>[2x]MANDSVSLTSNISNTSGVLLESQTKITDGALHFDGKKLNHNTFENPSKSQAYDYFFGRNISAHGDAVKPYKHFVFMTWYKGGKEERNVMLSRFNTKTGVVKTIQFPHRHTGFRGDPLVGESHNTIGLAVSPLNGTIHMVYDMHAYVDDDETGRFKGRFVDDFFRYSFSVAGAADVPDDEFTLEQFVKD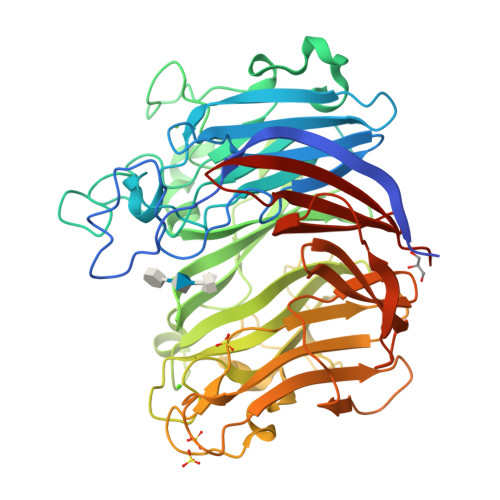TSELSQGADDYKHLTMTGNLQDKENFSALTYPKFYTSDDGELLHYMRWGGNNNGAYYFNKYDAKNQKWTRFTPFNHKDQKTHGNAYNWGLYGQMKYINGKLRVGFQQNSANNDDRFKYQNGVYYAYSDHPDGLGNWKNVDGEDMTWPLVNSDEIKIFEPGDYIDHTAPNSVHIVTGFDWTVTENDDVHFITHVRSTDTKRSDYKEVSIHAFKPANAVDFTITTDFTGADSIYTSGDSIFIIGLKNGYPFVEKAKGGSNDFEVVYQQASGVKFDHGTIHIENGKAYYYLMEKGAGNALPLHLQVIDLGVTELEHHHHHH> MKIAVIGQSLFGQEVYCQLRKEGHEVVGVFTIPDKDGKADPDGLEAEKDGVPVFKFPRWRARGQALPEVVAKYQALGAELNVLPFCSQFIPMEVINAPRHGSIIYHPSLLPRHRGASAINWTLIHGDKKGGFTIFWADDGLDTGDLL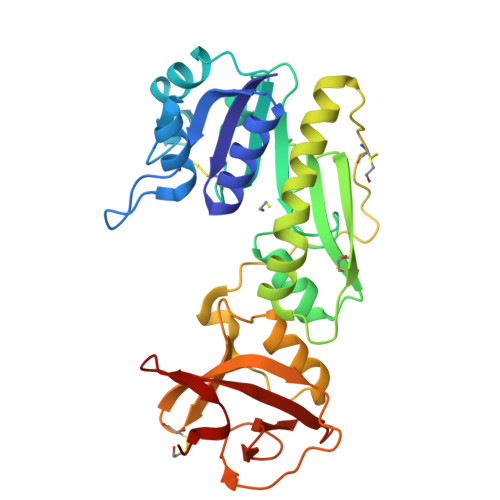LQKECEVLPDDTVSTLYNRFLFPEGIKGMVQAVRLIAEGTAPRCPQSEEGATYEGIQKKETAKINWDQPAEAIHNWIRGNDKVPGAWTEACGQKLTFFNSTLNTSGLSTQGEALPIPGAHRPGVVTKAGLILFGNDDRMLLVKNIQLEDGKMMPASQFFKGSD Macrophage migration inhibitory factor (MIF) is an inflammatory protein with various non-overlapping functions. Human MIF is a homotrimer with an enzymatic cavity between two subunits with Pro1 as a catalytic base, activates the receptors CD74, CXCR2, and CXCR4, has functional interactions in the cytosol, and is reported to be a nuclease. MIF forms a homotrimeric structure with a solvent channel coincident with its 3-fold axis and possesses three putative catalytic cavities formed at the interface between each of two adjacent subunits. Recently, we discovered an allosteric regulatory site at the center of the symmetric MIF homotrimer that serves as a hub for two of its biochemical activities: the enzymatic enol-keto tautomerase and CD74 receptor activation.

To investigate this relationship further, we introduced a cysteine residue at position 99 (Y99C). We hypothesized that this mutation would enable disulfide stabilized dimers within the MIF trimers, providing a more comprehensive understanding of the structural, dynamic, and functional impact of Cys99 substitution. The structure of homotrimeric Y99C MIF was solved to 1.60 Å to probe whether there were sufficient protein dynamics for the Cys99 side chain to form a disulfide and to detect any unexpected effects. The X-ray structure of the Y99C MIF homotrimer did not reveal the presence of a disulfide between any two of three subunits. From this alignment, the residue 99 sidechains indicate the Cβ carbons overlap very well. Interestingly, the thiol group in all three monomers has two conformations in the channel as shown in Figure 3A where Y99 and Y99A are also shown. The closest distances among the thiol groups of adjacent subunits are ∼6.5 Å. The two conformations of the thiol groups in this study do not interact with other protein atoms nor do they induce large conformational changes. Though the shared Cβ atom for WT, Y99A, Y99C MIF align very well, the radius of the solvent channel opening where the three Y99C residues appear is 3.4 Å and similar to Y99A (3.6 Å), in contrast to WT MIF (1.4 Å) as calculated by MOLEonline. Though we observed a solvent channel opening for Y99C similar to that of Y99A, the catalytic activity of the Y99C homotrimers has reduced (55%) catalytic efficiency relative to WT MIF and compared to Y99A (77%). The Y99C homotrimer abolished CD74 activation in vivo but possessed reduced enzymatic activity, supporting the role of Tyr99 as a common allosteric node within two distinct allosteric pathways.

>[3x]PMFIVNTNVPRASVPDGFLSELTQQLAQATGKPPQYIAVHVVPDQLMAFGGSSEPCALCSLHSIGKIGGAQNRSYSKLLCGLLAERLRISPDRVYINYCDMNAANVGWNNSTFA> TGTAGDLASLLAGDGLGRKSKAWRVLRAQQQACGEGSGEEGEITEIEGLGLGEGMEGFERELDNIPDTLPDDERLALWKGKLKHYLILSSAGKPIWSRHGDLSLVNSTMGVVQTIISFYEGARNPLLGFTAGKVRFVILIKGPLYFVAISRLRESDAQLRAQLEALYMQILSTLTLPILTNIFAHRPSTDLRGPLQGTESLLASLADSFTKGSPSTLLSALECLRLRKSQRQAITNIFLKSRCEELLYGLLVAGGKLVSVIRPRKHSLHPSDLQLIFNMLFESGGIKGNGGENWIPLCLPAFNNTGYLYMYVSFLDDKAPDDQNQPPESSNLDASNKNSSNTPDDDLTALILISPSREAFYALQSMRTRLVSQLLSTGYLSLIRSTALSGRPSITSILPKTPLLHFLYKSRPNVQWCMSSLSSLTPPGATATETLLARRKLMSVYEELHA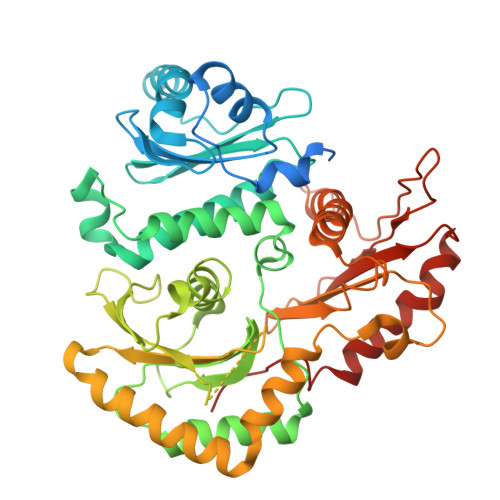ALHARHAHLRVVYSTADEKEGEGLACLGWSTPAFEVYCVAPGCVGRAGMAREVNRVVQWARREEERLFILGGGVF> APSYPEYTREEVGRHRSPEERVWVTHGTDVFDVTDFVELHPGGPDKILLAAGGALEPFWALYAVHGEPHVLELLQQYKVGELSPDEAPAAPDAQDPFAGDPPRHPGLRVNSQKPFNAEPPAELLAERFLTPNELFFTRNHLPVPAVEPSSYRLRVDGPGGGTLSLSLAELRSRFPKHEVTATLQCAGNRRSEMSRVRPVKGLPWDIGAISTARWGGARLRDV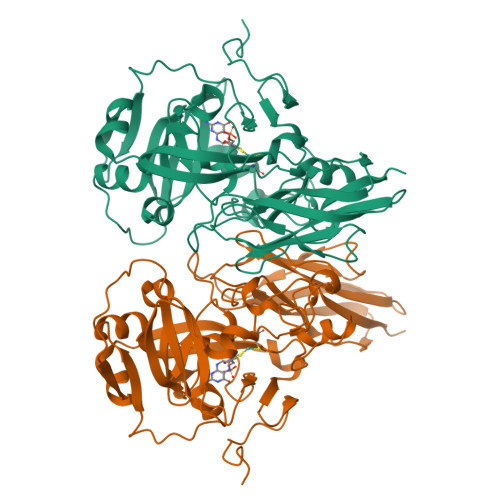LLHAGFPEELQGEWHVCFEGLDADPGGAPYGASIPYGRALSPAADVLLAYEMNGTELPRDHGFPVRVVVPGVVGARSVKWLRRVAVSPDESPSHWQQNDNKGFSPCVDWDTVDYRTAPAIQELPVQSAVTQPRPGAAVPPGELTVKGYAWSGGGREVVRVDVSLDGGRTWKVARLMGDKAPPGRAWAWALWELTVPVEAGTELEIVCKAVDSSYNVQPDSVAPIWNLMGVLSTAWHRVRVSVQD>AERTGLKATAWKPLCKLTTELSKVSGEMLNEGQEVISNIQKIKAAEY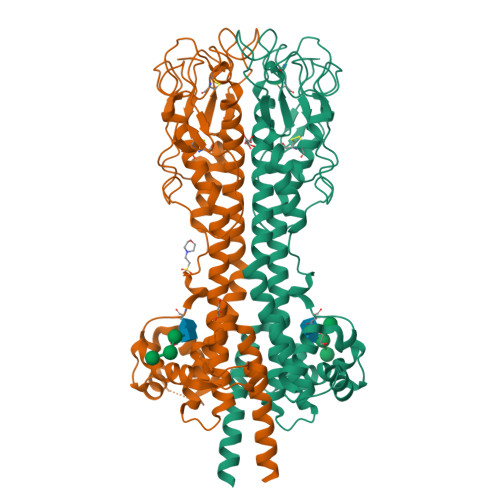KVSIYLAKNPETQALQQLTLLRGYFARKTNGGLESYKTMGLATQIRSARAAAYLKGSIDEFLNLLESLKGGSENKCLVTTNADTAATRRETKLDDQECALSMPETKPEAATRTELTQTGYPNLQHGGGGTANTFQPTTSTGTCKLLSGHSTNGYPTTSALDTTAKVLAGYMTIPNTQVEATLANMQAMGNGHKATAPAWHEAWEARNREAKAKDLAYTNETGNLDTQPTLKALVKTLLLPKDNTEHNAEATKLEALFGGLAADKTKTYLDMVDAEIIPAGIAGRTTEAPLGKIHDTVELGDILSNYEMIAAQNVVTLKKNL[2x]>[2x]MTSCHIAEEHIQK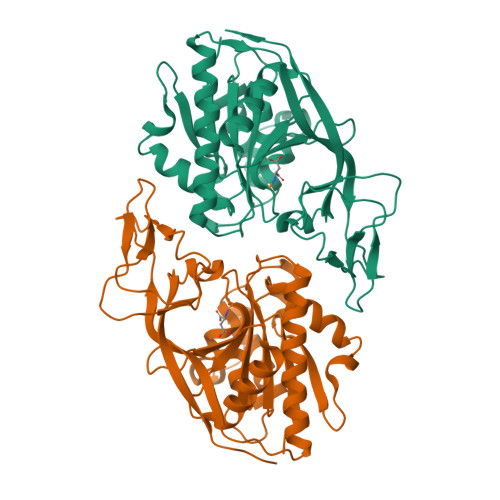VAIFGGTHGNELTGVFLVKHWLENGAEIQRTGLEVKPFITNPRAVKKCTRYIDCDLNRIFDLENLGKKMSEDLPYEVRRAQEINHLFGPKDSEDSYDIIFDLHNTTSNMGCTLILEDSRNNFLIQMFHYIKTSLAPLPCYVYLIEHPSLKYATTRSIAKYPVGIEVGPQPQGVLRADILDQMRKMIKHALDFIHHFNEGEEFPPCAIEVYKIIEKVDYPRDENGEIAAIIHPNLQDQDWKPLHPGDPMFLTLDGKTIPLGGDCTVYPVFVNEAAYYEKKEAFAKTTKLTLNAKSIRCCLH>[2x]MAHHHHHHVDDDDKMVHHDGFQTVKATIDWEHPMFKLYEKAKRNGKWNPADIDFSQDQKDFASLTSEEKISALPLVAGFSAGEEALTLDILPMAHALARQGRLEDVLFLTTFMHDEAKHVEMFSRWQQAVGIGQMDLSVFHNDHYKRIFYEALPEAMNRLYADDSPEAVIRAATVYNMIVEGTLAESGYYTFRQIYKKAGLFPGLLQGIDYLNMDEGRHIQFGIYTIQRIVNEDERYYELFIRYMDELWPHVIGYVDYLTELGKRQQQLARTYALEIDYDLLRHYVIKQFNLRKKQISRTKRVDVVEGLEKTAAES

The heterodinuclear Mn/Fe cofactor is found in the R2 subunits of subclass Ic ribonucleotide reductases (denoted as R2c) as well as a related group of proteins known as R2-like ligand-binding oxidases (R2lox). Although the physiological function of R2lox proteins is not known, the cofactor catalyzes formation of a tyrosine–valine ether cross-link in the protein scaffold. Two proteins from this group have been characterized to date, homologs from Mycobacterium tuberculosis and Geobacillus kaustophilus. Both contain the ether cross-link, and both co-purify from heterologous expression hosts with a long-chain fatty acid ligand bound in a hydrophobic channel leading from the protein surface to the active site, hence the name ligand-binding oxidase. The two metal ions are bound next to each other in octahedral geometry by two histidines and four glutamates, with the manganese ion occupying the N-terminal metal-binding site 1.

The cross-linking valine, which is completely conserved across the R2lox group, was changed to an alanine, isoleucine or leucine (V72A/I/L). Crystal structures were obtained of all three R2lox point mutants in the non-activated reduced and the oxidized resting state by soaking apo-protein crystals with MnII and FeII under anoxic or aerobic conditions, respectively. The V72A/L mutations were found to have little effect on the global structures of the reduced and oxidized resting states, but an ether cross-link was not formed in the oxidized state. In the wild-type, the hydroxyl group of Y162 is hydrogen-bonded to the carbonyl oxygen of V72 prior to cross-link formation, and this hydrogen bond is maintained in V72A/L-R2lox in the oxidized state. In the oxidized state, it appears that the bridging fatty acid ligand is slightly tilted towards residue 72 in V72A- and away from it in V72L-R2lox, although these slight differences are within the range of the coordinate error. More mass spectrometry samples were consequently prepared in the dark. The Y162-I72 cross-linked peptide was obtained by digestion of aerobically Mn/Fe-reconstituted V72I-R2lox, but only if the samples were processed in the dark, whereas the cross-link was not present in V72L-R2lox (Fig. S1 and data not shown). The Mn/Fe cofactor can thus oxidize the tertiary carbon of a valine or isoleucine, but not that of a leucine, indicating that the carbon atom has to be in the correct relative position to the metal center to be oxidized. Moreover, only a tertiary beta-carbon of residue 72 is oxidized by R2lox, as the tertiary gamma-carbon of a leucine in position 72 is not.>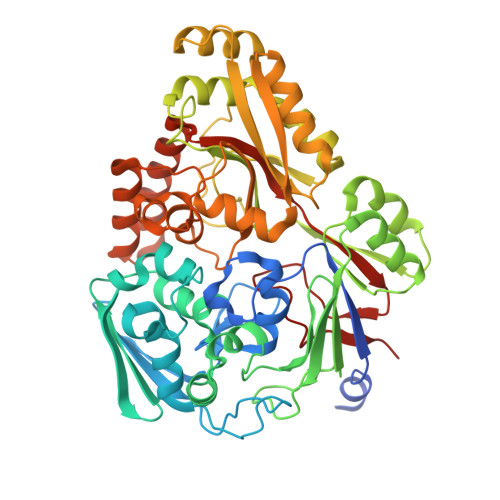 GIDPFTSENPNATLNPSKENISVKEQKRFGGVLVFARGADGSSMDPALVTDGESYVATGNIYDTLVQFKYGTTEIEPALATSWDISPDGLVYTFHLRKGVYFHQTKYWNKKVEFSAKDVLFSFERQMDKAKRYYSPGAKSYKYWEGMGMSHIIKSIEALDDYTIRFTLNGPEAPFLANLGMDFLSILSKDYADYLEQNNKKDELAKKPVGTGPFKFFLWNKDEKIILLKNQDYWGPKAYLDKVVVRTIPNSSTRALALRTGEIMLMTGPNLNEVEQLEKLPNIVVDKSAGLLASWLSLNTQKKYFNNPLVRLAINHAINVDDYIKVIYEGFAQKMVNPFPPTIWGYNYNIKPYEYDLKKAKELLKQAGYPNGFKTTIFTTSTRNPKGAVFIQASLAKIGIDVKIEVYEWGAYLKRTGLGEHEMAFAGWMADIADPDNFLYTLWSKQAASAIPTQNGSFYKSDAFSDLLIKAKRVSDQKEREALYLKAQEIIHKDAPYVPLAYPYSVVPHLSKVKGYKTTGVSVNRFFKVYLEK>MRILVIEDEISLNKTIIDNLNEFGYQTDSSENFKDGEYFIGIRHYDLVLASWNLPDGDGAELVNTIKHKSPRTSVMIMSAKADKDTEIKALKAGADDFVKKPLDFDILLARIEARLRLGGTNVIKIEDLVIDPDEEKITYKGQDIELKGKPFEVLTHLARHSDQIVSKEQLLDAIWEEPELVTPNVIEVAINQIRQKMDKPLNISTIETVRRRGYRFCFPKKS[2x]

The C. jejuni CosR regulator is essential to the viability of this bacterium and is responsible for regulating the expression of a number of oxidative stress defense enzymes. Importantly, it also modulates the expression of the CmeABC multidrug efflux system, the most predominant and clinically important system in C. jejuni that mediates resistance to multiple antimicrobials. CosR belongs to an OmpR/PhoB family of response regulators. We determined that CosR assembles as a homodimer with each CosR protomer contributing to major conformational changes to facilitate DNA binding.

Next, 8 mg/mL of purified full-length CosR was mixed with 2.6 mg/mL of 21 bp double-stranded DNA1, which contains two half-sites, S1 and S2, for dimeric CosR binding, and crystallization trials were again conducted. The best crystal of the CosR-DNA1 complex diffracted X-rays to 2.90 Å. Each unit cell of the CosR-DNA1 crystal contains two CosR protomers and one DNA duplex. One of the CosR protomers is bound at S1 of one DNA chain. The other CosR protomer in the unit cell is associated with S2 of the DNA chain. Superimposition of these two CosR protomers gives rise to a very high root-mean-square deviation (r.m.s.d.) of 9.5 Å, suggesting that they are structurally very distinct from each other. The CosR protomer, designated CosR1, bound by the S1 site, has an elongated and extended conformation. However, the other CosR protomer that contacts the S2 site, designated CosR2, has a more compact conformation. However, by applying a crystallographic symmetry operator, it is found that CosR1 and CosR2 indeed tightly contact with each other and assemble as an asymmetric dimer to bind the DNA duplex. Interestingly, this CosR dimer appears to hold the two DNA1 chains together, where the two DNA1 align in such a way that the tail of the first chain contacts the head of the second chain.>MPSITFIHPDGRSEIVDAAIGDSAMFAALNHGIDSIVAECGGNAVCATCHVYVDDLWLAKLPPVDANEDDLLDGTASDRLPNSRLSCQIKIAPELDGLVLRI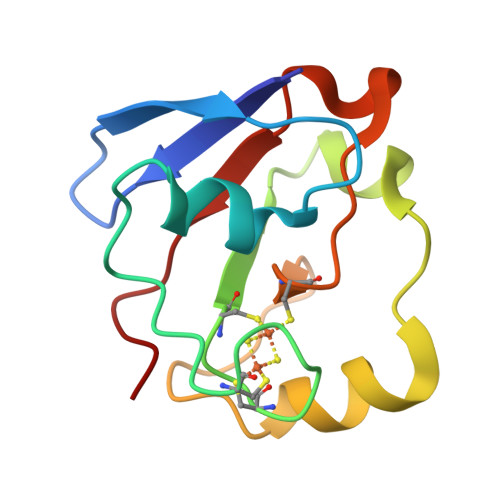PERQT[2x]>[2x]MSEITLGKYLFERLKQVNVNTVFGLPGDFNLSLLDKIYEVEGMRWAGNANELNAAYAADGYARIKGMSCIITTFGVGELSALNGIAGSYAEHVGVLHVVGVPSISSQAKQLLLHHTLGNGDFTVFHRMSANISETTAMITDIATAPAEIDRCIRTTYVTQRPVYLGLPANLVDLNVPAKLLQTPIDMSLKPNDAESEKEVIDTILALVKDAKNPVILADACCSRHDVKAETKKLIDLTQFPAFVTPMGKGSISEQHPRYGGVYVGTLSKPEVKEAVESADLILSVGALLSDFNTGSFSYSYKTKNIVEFHSDHMKIRNATFPGVQMKFVLQKLLTNIADAAKGYKPVAVPARTPANAAVPASTPLKQEWMWNQLGNFLQEGDVVIAETGTSAFGINQTTFPNNTYGISQVLWGSIGFTTGATLGAAFAAEEIDPKKRVILFIGDGSLQLTVQE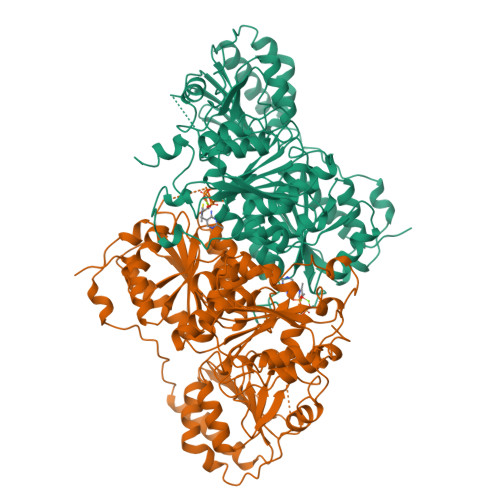ISTMIRWGLKPYLFVLNNDGYTIEKLIHGPKAQYNEIQGWDHLSLLPTFGAKDYETHRVATTGEWDKLTQDKSFNDNSKIRMIEIMLPVFDAPQNLVKQAKLT>MRKVIIKENPSEE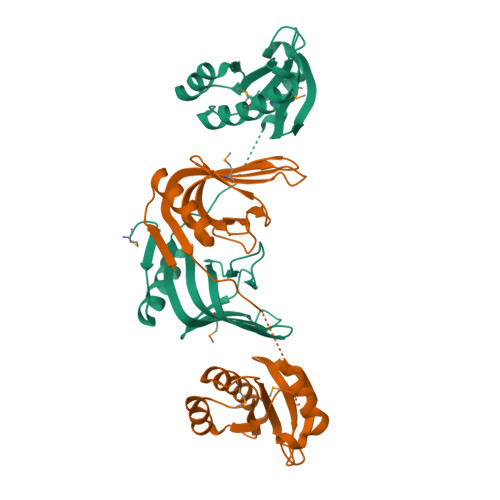EIKELLDLAEKHGGVVTIFARCKVHYEGRAKSELGEGDRIIIIKPDGSFLIHQNKKREPVNWQPPGSKVTFKENSMISIRRRPYERLEVEIIEPYSLVVFLAEDYEELALTGSEAEMANLIFENPRVIEEGFKPIYREKPIRHGIVDVMGVDKDGNIVVLELKRRKADLHAVSQMKRYVDSLKEEYGENVRGILVAPSLTEGAKKLLEKEGLEFRKLEPPKKGNEKRSKQKTLDFFTP[2x]> GSGGSGMIPYQEWHSQLQSLYDSQIFHNWALSQDVHLNDEKDGLLLRLIPTRQLQKNTERIENKLLNHIELYLTYSKVYNEPLLLLRIWEEKSIDGIPMTKLMLPTDIESLLDVQGKFQLGLDTIINLEGSVWYSFHPCD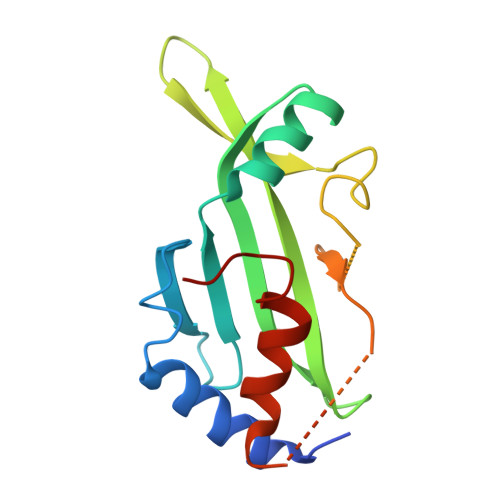TSSIVGDQAEFMSTYLRRWVSIFIFSWLGYEDS> MPAEITSLPLFPLHSVLLPGATIGLRVFERRYLDLVRDCGRTGSSFGVCLILDGS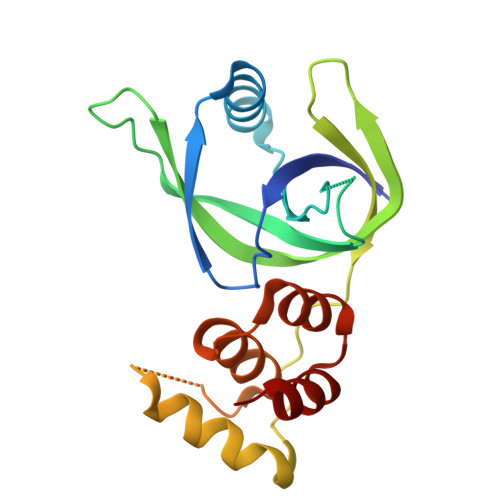DVGAPAVPAAYGTEVRIEDFDVGNDGVLVLRLRGTRRFRVQRSRVRDNGLVVGEVSWCEPDSDDELRPEHGLLATVLERMLEQVGGEFASAGPGLLDQAAWVGWRLAELLPLSEGQRLSLLQEDDPHRRLEQLLAWMP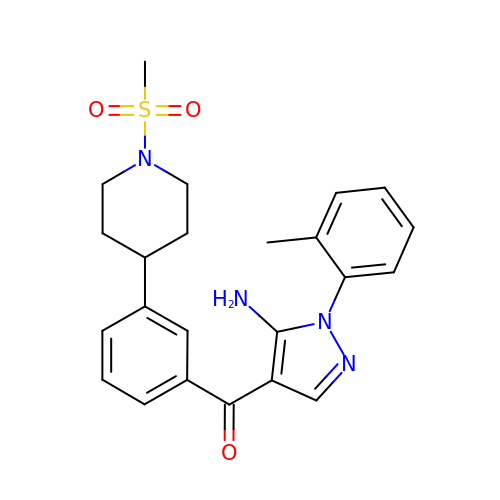[5-amino-1-(2-methylphenyl)-1H-pyrazol-4-yl]{3-[1-(methylsulfonyl)piperidin-4-yl]phenyl}methanone | C23 H26 N4 O3 S | KOCQZKPUMDARNV-UHFFFAOYSA-N> VRLPGLAAMRQGTRLFTPEQGEDLREALRRRRGSFQTTCEVTSETTFAAARRLREKASALAALNFASAKNPGGGFLGGAQAQEEDLCRGSGLYFSLTSPQAEPYYAVNRQSHSALYTDHLIYSPQVPIFRDDAGQLLPAPVPVNIITAPAPNAGAVAQSRPEQLPQVLPTLRERA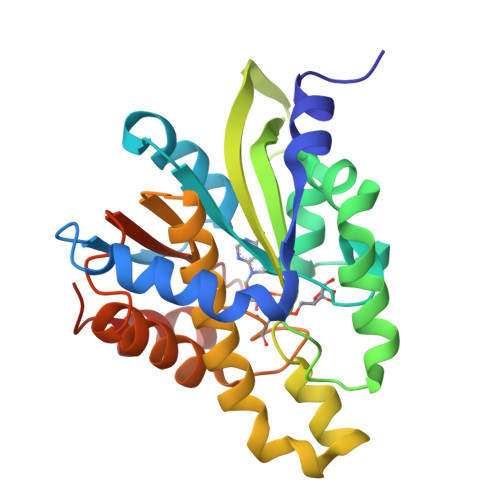RRVLGVAAWMEQTHLVLGAWGCGVFRNDPAGVARTFRELLEGEAQGAFEHVTFAVLDNHPQHPRLGAFRRELESLC>[5x]TVTYTNRVADARLGTFSQLLLQWKGSIYKLLYSEFLIFISLYFAISLVYRLILSESQRLMFEKLALYCNSYAELIPVSFVLGFYVSLVVSRWWAQYESIPWPDRIMNLVSCNVDGEDEYGRLLRRTLMRYSNLCSVLILRSVSTAVYKRFPSMEHVVRAGLMTPEEHKKFESLNSPHNKF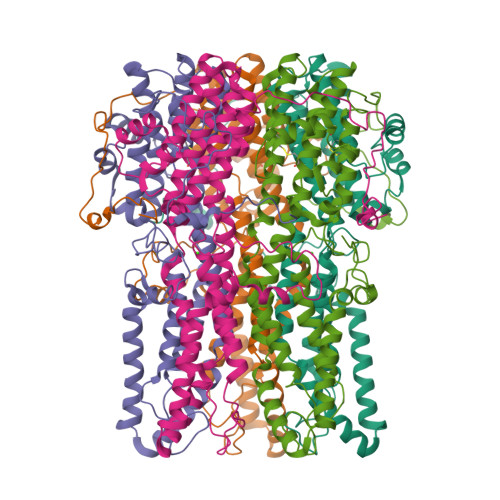WIPCVWFSNLAVKARNEGRIRDSVLLQGILNELNTLRSQCGRLYGYDWISIPLVYTQVVTVAVYSFFLACLIGRQFLDPEKAYPGHELDLFVPVFTFLQFFFYAGWLKVAEQLINPFGEDDDDFETNWLIDRNLQVSLMAVDEMHQDLPILEKDLYWNEPDPQPPYTAATAEYKRPSFLGSTFDISMQKEEMEFQPLEQIKENEEANHSTPLLGHLGRLLGVQSEGEEF> SADAQSFLNRVCGVSAARLTPCGTGTSTDVVYRAFDIYNDKVAGFAKFLKTNCCRFQEKDEDDNLIDSYFVVKRHTFSNYQHEETIYNLLKDCPAVAKHDFFKFRIDGDMVPHISRQRLTKYTMADLVYALRHFDEGNCDTLKEILVTYNCCDDDYFNKKDWYDFVENPDILRVYANLGERVRQALLKTVQFCDAMRNAGIVGVLTLDNQDLNGNWYDFGDFIQTTPGSGVPVVDSYYSLLMPILTLTRALTAESHVDTDLTKPYIKWDLLKYDFTEERLKLFDRYFKYWDQTYHPNCVNCLDDRCILHCANFNVLFSTVFPPTSFGPLVRKIFVDGVP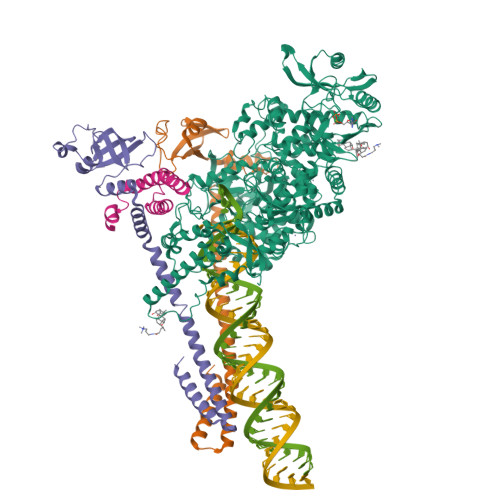FVVSTGYHFRELGVVHNQDVNLHSSRLSFKELLVYAADPAMHAASGNLLLDKRTTCFSVAALTNNVAFQTVKPGNFNKDFYDFAVSKGFFKEGSSVELKHFFFAQDGNAAISDYDYYRYNLPTMCDIRQLLFVVEVVDKYFDCYDGGCINANQVIVNNLDKSAGFPFNKWGKARLYYDSMSYEDQDALFAYTKRNVIPTITQMNLKYAISAKNRARTVAGVSICSTMTNRQFHQKLLKSIAATRGATVVIGTSKFYGGWHNMLKTVYSDVENPHLMGWDYPKCDRAMPNMLRIMASLVLARKHTTCCSLSHRFYRLANECAQVLSEMVMCGGSLYVKPGGTSSGDATTAYANSVFNICQAVTANVNALLSTDGNKIADKYVRNLQHRLYECLYRNRDVDTDFVNEFYAYLRKHFSMMILSDDAVVCFNSTYASQGLVASIKNFKSVLYYQNNVFMSEAKCWTETDLTKGPHEFCSQHTMLVKQGDDYVYLPYPDPSRILGAGCFVDDIVKTDGTLMIERFVSLAIDAYPLTKHPNQEYADVFHLYLQYIRKLHDELTGHMLDMYSVMLTNDNTSRYWEPEFYEAMYTPHTVLQ;>MAIASEFSSLPSYAAFATAQEAYEQAVANGDSEVVLKKLKKSLNVAKSEFDRDAAMQRKLEKMADQAMTQMYKQARSEDKRAKVTSAMQTMLFTMLRKLDNDALNNIINNARDGCVPLNIIPLTTAAKLMVVIPDYNTYKNTCDGTTFTYASALWEIQQVVDADSKIVQLSEISMDNSPNLAWPLIVTALRANSAVKLQ[2x];> GPVDMSKMSDVKCTSVVLLSVLQQLRVESSSKLWAQCVQLHNDILLAKDTTEAFEKMVSLLSVLLSMQGAVDINKLCEEMLDNRATLQ methyl 2-(hydroxymethyl)-6~{H}-thieno[2,3-b]pyrrole-5-carboxylate | C9 H9 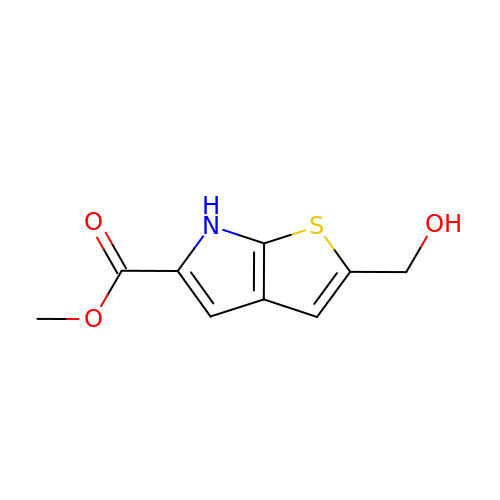N O3 S | FJDCCIDVLHNLOW-UHFFFAOYSA-N>G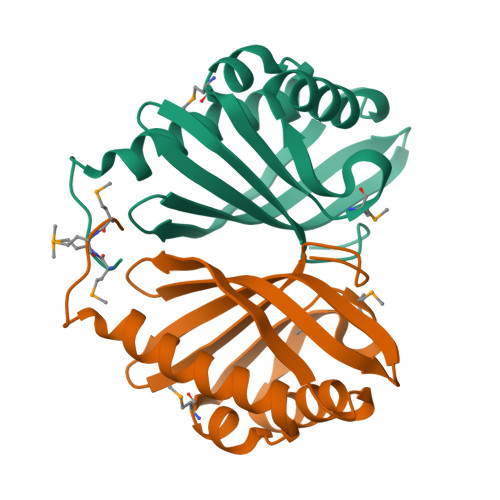MMTHYSDNTLKVAHQGFEFFTQGLATGEWQKFLDMLTEDFTFWFPMGEFHGLNVGKERAKEFFTYVSESFHTGIQISSLDRVTSNETTVVFEFRDEGLFLGKPYKNRVAVSFDVRGDKICSYREYFGSDGKSN[2x]> MQTSARNQWFGTITARDHDDVQQHVDVLLADGKTRLKVAITAQSGARLGLDEGKEVLILLKAPWVGITQ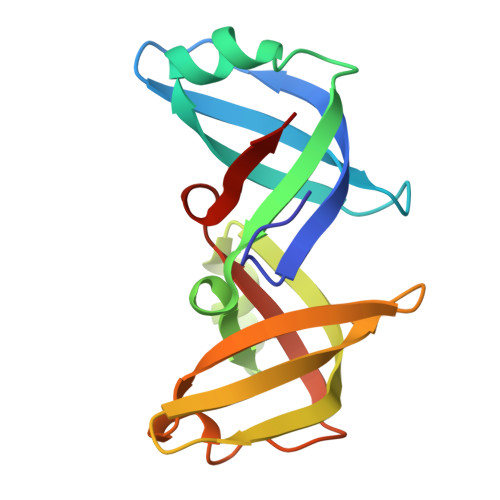DEAVAQNADNQLPGIISHIERGAEQCEVLMALPDGQTLCATVPVNEATSLQQGQNVTAYFNADSVIIATLC> GSHMEAVQNRIVEAAERVPGVRGVIHLRARYVGQDIWADMIIGVDPENTVE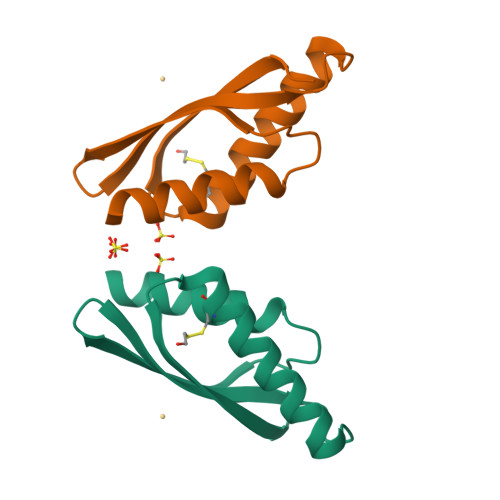QAHEICEAVQAAVCGKIRRIESLDVSAEAREIGDTTKPSFSDQPLSFDEVMLSKVDN> MSNFKV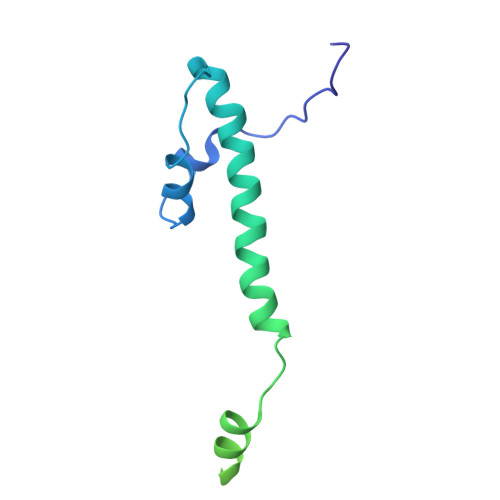RDPVIQERLDHDYAHHPLVARMNTLDQGNMSQAEYLVQKRHYLVFLIAHHYYEAYLRRMGGIQRRDHLQTLRDQKPRERADRVSAASAYDAGTFTVPSRPGPASGTTPGGQDSLGVSGSSITTLSSGPHSLSPASDILTTLSSTTETAAPAVADARKPPSGKKK> MHHHHHHELENYEQPVVLREDNRRRRRRMKPRSTAASLSSMELIPIEFVLPTSQRNTKTPETALLHVAGHGNVEQMKAQVWLRALETSVSADFYHRLGPDHFLLLYQKKGQWYEIYDKYQVVQTLDCLRYWKVLHRSPGQIHVVQRHAPSEETLAFQRQLNALIGYDVTDVSNVHDDELEFTRRRLVTPRMAEVAGRDPKLYAMHPWVTSKPLPEYLLKKITNNCVFIVIHRSTTSQTIKVSADDTPGTILQSFFTKMAKKKSLMDIPESQNERDFVLRVCGRDEYLVGETPIKNFQWVRQCLKNGEEIHLVLDTPPDPALDEVRKEEWPLVDDCTGVTGYHEQLTIHGKDHESVFTVSLWDCDRKFRVKIRGIDIPVLPRTADLTVFVEANIQYGQQVLCQRRTSPKPFTEEVLWNVWLEFSIKIKDLPKGALLNLQIYCGKAPALSGKTSAEMPSPESKGKAQLLYYVNLLLIDHRFLLRHGEYVLHMWQLSGKGEDQGSFNADKLTSATNPDKENSMSISILLDNYCHPIALPKHRPTPDPEGDRVRAEMPNQLRKQLEAIIATDPLNPLTAEDKELLWHFRYESLKDPKAYPKLFSSVKWGQQEIVAKTYQLLAKREVWDQSALDVGLTMQLLDCNFSDENVRAIAVQKLESLEDDDVLHYLLQLVQAVKFEPYHDSALARFLLKRGLRNKRIGHFLFWFLRSEIAQSRHYQQRFAVILEAYLRGCGTAMLHDFTQQVQVIDMLQKVTIDIKSLSAEKYDVSSQVISQLKQKLENLQNLNLPQSFRVPYDPGLKAGALVIEKCKVMASKKKPLWLEFKCADPTALSNETIGIIFKHGDDLRQDMLILQIL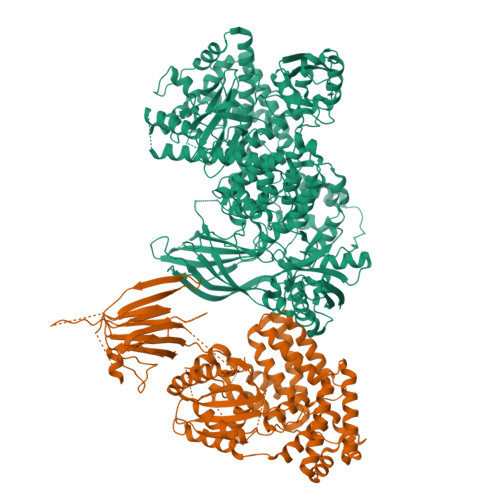RIMESIWETESLDLCLLPYGCISTGDKIGMIEIVKDATTIAKIQQSTVGNTGAFKDEVLSHWLKEKCPIEEKFQAAVERFVYSCAGYCVATFVLGIGDRHNDNIMISETGNLFHIDFGHILGNYKSFLGINKERVPFVLTPDFLFVMGTSGKKTSLHFQKFQDVCVKAYLALRHHTNLLIILFSMMLMTGMPQLTSKEDIEYIRDALTVGKSEEDAKKYFLDQIEVCRDKGWTVQFNWFLHLVLGIKQGEKHSA;> MQPGATTCTEDRIQHALERCLHGLSLSRRSTSWSAGLCLNCWSLQELVSRDPGHFLILLEQILQKTREVQEKGTYDLLAPLALLFYSTVLCTPHFPPDSDLLLKAARTYHRFLTWPVPYCSICQELLTFIDAELKAPGISYQRLVRAEQGLSTRSHRSSTVTVLLLNPVEVQAEFLDVADKLSTPGPSPHSAYITLLLHAFQATFGAHCDLSGLHRRLQSKTLAELEAIFTETAEAQELASGIGDAAEARQWLRTKLQAVGEKAGFPGVLDTAKPGKLRTIPIPVARCYTYSWNQDSFDILQEILLKEQELLQPEILDDEEDEDEEDEEEDLDADGHCAERDSVLSTGSAASHASTLSLASSQASGPTLSRQLLTSFVSGLSDGVDSGYMEDIEESAYERPRRPGGHERRGHRRPGQKFNRIYKLFKSTSQMVLRRDSRSLEGSPDSGPPLRRAGSLCSPLDSPTLPPSRAQRSRSLPQPKLSPQLPGWLLAPASRHQRRRPFLSGDEDPKASTLRVVVFGSDRISGKVARAYSNLRRLENNRPLLTRFFKLQFFYVPVKRSRGTGTPTSPAPRSQTPPLPTDAPRHPGPAELGAAPWEESTNDISHYLGMLDPWYERNVLGLMHLPPEVLCQSLKAEPRPLEGSPAQLPILADMLLYYCRFAARPVLLQVYQTELTFITGEKTTEIFIHSLELGHSAATRAIKASGPGSKRLGIDGDREAVPLTLQIIYSKGAISGRSRWSNMEKLCTSVNLSKACRQQEELDSSTEALTLNLTEVVKRQTPKSKKGFNQISTSQIKVDKVQIIGSNSCPFAVCLDQDERKILQSVIRCEVSPCYKPEKSSLCPPPQRPSYPPAPATPDLCSLLCLPIMTFSGALPGGGGSDYKDDDDK>STQAAPLISVEKIQKLAQSYQGDTRKRFTAWGNLIDSLKKKPVKIQLEKVNSFFNQFNYETDPITGASDDYWKSPVEFIVDGGGDCEDFAIIKYFTLVAVGVPSDQLRITYAASLTLNQAHMVLSFYPTPESEPLILDSLESKILKASARPDLKPVYSFNAEGLWLAKTRGESSLMGDSK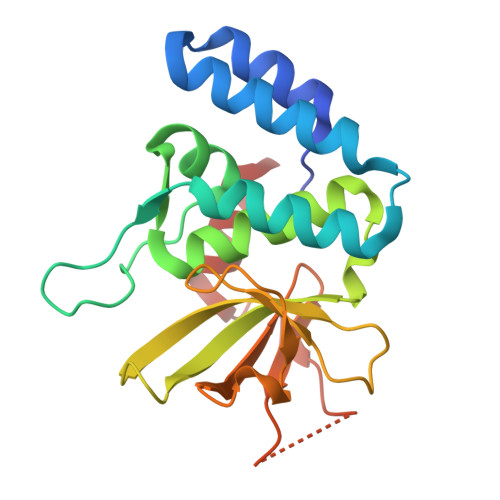SLGKWDALMKRME[2x]N-(2,4-di-tert-butyl-5-hydroxyphenyl)-4-oxo-1,4-dihydroquinoline-3-carboxamide | C24 H28 N2 O3 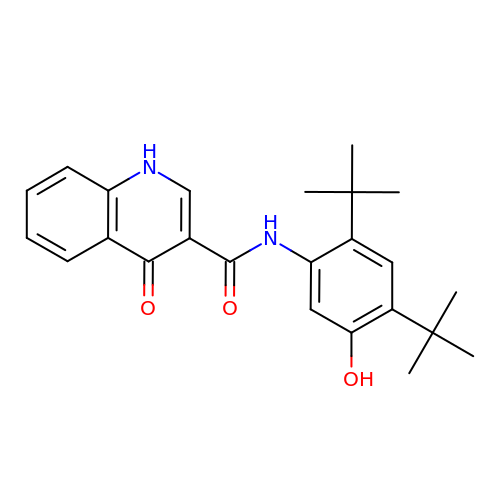| PURKAOJPTOLRMP-UHFFFAOYSA-N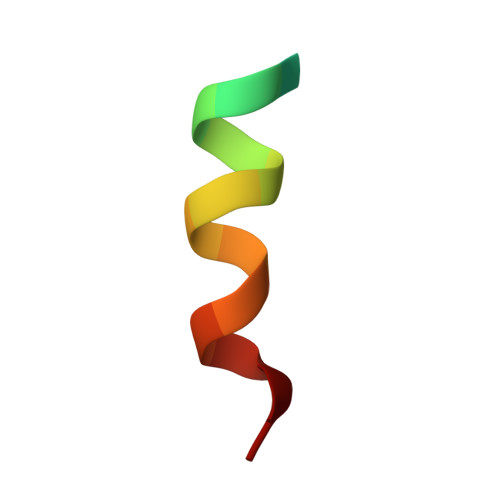> EQKSDEETKKNAMKLIN HAdV-D10 is a rare serotype isolated from the eyes of patients with conjunctivitis. HAdV are non-enveloped viruses measuring 90–100 nm and arranged in an icosahedral capsid with protruding fiber proteins at the pentameric vertices. Structural and biological studies of HAdV-D10 knob protein highlighted low-affinity engagement with native adenoviral receptors CAR and sialic acid. HAdV-D10 possesses characteristics of a promising virotherapy, combining low seroprevalence, weak receptor interactions, and reduced off-target uptake.

Taking all together, we generated the first reported structure of the HAdV-D10 fiber knob and demonstrated that HAdV-D10K can form weak interactions with several known adenoviral receptors and may use CAR and/or sialic acid for infection. We investigated binding of HAdV-D10K to known adenoviral receptors CAR, CD46, and DSG2 by using surface plasmon resonance. HAdV-D10K was able to bind to all three receptors, but the interaction was weak for CD46 and DSG2 (KD: 20 and 125 μM). We demonstrated that HAdV-D10K forms a stronger interaction with CAR than CD46 and DSG2 (0.44 μM). This is still considered a weak interaction in comparison with CAR binding to HAdV-C5 knob (0.76nM). We conclude that, although the binding is weak, HAdV-D10 can bind and use CAR as an entry receptor. Although several binding sites were identified, we determined that HAdV-D10K forms weak interactions with CD46, insufficient for cell entry.

>MRGHHHHHHGSGDLVAWNVKHDTRTLWTTPDTSPNCTIAQDKDSKLTLVLTKCGSQILANVSLIVVAGKYHIINNKNNPEIKSFTIKLLFDKNGVLLDNSNLGKTYWNFRSGDSNVSTAYEKAIGFMPNLVAYPKPSNSKKYARDIVYGTIYLGGKPDQPAVIKTTFNQETGCEYSITFDFSWSKTYENVEFETTSFTFSYIAQQ[6x]> SMSKNNIFNKYPTIIHGEARGENDEFVVHTRYPRFLARKSFDDNFTGEMPAKPVN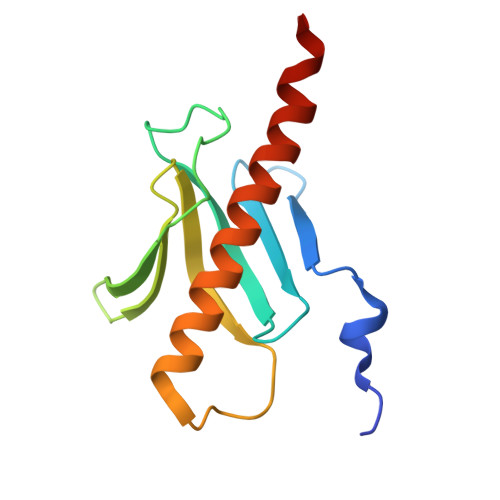GELGQIGEPRRLAYDSRLGLWLSDFIMLDNNKPKNMEDWLGQLKAACDRIAADDLMLNEDAADLEGWDD>MASMTGGQQMGRGSMSRDPLPFFPPLYLGGP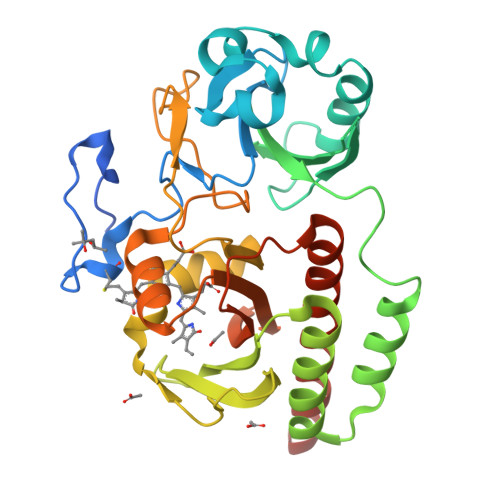EITTENCEREPIHIPGSIQPHGALLTADGHSGEVLQMSLNAATFLGQEPTVLRGQTLAALLPEQWPALQAALPPGCPDALQYRATLDWPAAGHLSLTVHRVGELLILEFEPTEAWDSTGPHALRNAMFALESAPNLRALAEVATQTVRELTGFDRVMLYKFAPDATGEVIAEARREGLHAFLGHRFPASDIPAQARALYTRHLLRLTADTRAAAVPLDPVLNPQTNAPTPLGGAVLRATSPMHMQYLRNMGVGSSLSVSVVVGGQLWGLIACTHQTPYVLPPDLRTTLEYLGRLLSLQVQVKEALEHHHHHH[2x]Purine nucleoside phosphorylases (PNP, E.C. 2.4.2.1.) are ubiquitous enzymes of the purine salvage pathway enabling the cell to recover purine bases and ribose-1-phosphate from used purine nucleotides. PNPs catalyse the following reaction: β-purine nucleoside + orthophosphate ↔ purine base + α-D-pentose-1-phosphate. E. coli purine nucleoside phosphorylase is a homohexamer, which structure, in the apo form, can be described as a trimer of dimers. Dimers, but not monomers, seem to have all the necessary features to conduct catalysis, because monomers within a dimer mutually donate two amino acids to complete the active site of the neighbour.

First, a single-tryptophan Y160W mutant was engineered, with the mutation in a close proximity to the active site, but without significant interactions with ligands. Since each subunit of the wild type PNP contains six tyrosine residues and no tryptophan, this approach resulted in a protein with a significantly enhanced fluorescence response to ligand binding, and with retained catalytic and kinetic properties of the WT enzyme. The structure of the ternary complex of the Y160W mutant with sulfate and formycin A described in this study has a nucleoside bound only in two active sites per hexamer, located in the neighbouring subunits, but not belonging to the same dimer. Complex crystallised in P 6122 space group with the half of the hexamer in the asymmetric unit. Since phosphate was not present during the crystallisation, all active sites are in the open conformation. Moreover, even in these active sites the ligand is not bound in all protein molecules, since the occupancy of the formycin A molecule was found to be 0.71. The position of formycin A in the active site of the Y160W mutant, in the structure presented in this study is virtually the same as in the active site of the WT protein. Sulfate ion is bound in the hydrogen bond distance from Arg87, Arg43* (from the neighbouring subunit), Ser90, Gly20. Ribose of formycin A is involved in hydrogen bonds with sulfate ion, Glu181 and His4* (from the neighbouring subunit), whereas aglycon—with Asp204 and Ser90. The distribution of the nucleoside molecules in the Y160W enzyme subunits indicates that although all active sites are in the same open conformation, they do not share the same affinity to the ligand and are therefore not equivalent.

>ATPHINAEMGDFADVVLMPGDPLRAKYIAETFLEDAREVNNVRGMLGFTGTYKGRKISVMGHGMGIPSCSIYTKELITDFGVKKIIRVGSCGAVLPHVKLRDVVIGMGACTDSKVNRIRFKDHDFAAIADFDMVRNAVDAAKALGIDARVGNLFSADLFWSPDGEMFDVMEKYGILGVEMEAAGIYGVAAEFGAKALTICTVSDHIRTHEQTTAAERQTTFNDMIKIALESVLLGDK[3x]> MKKEK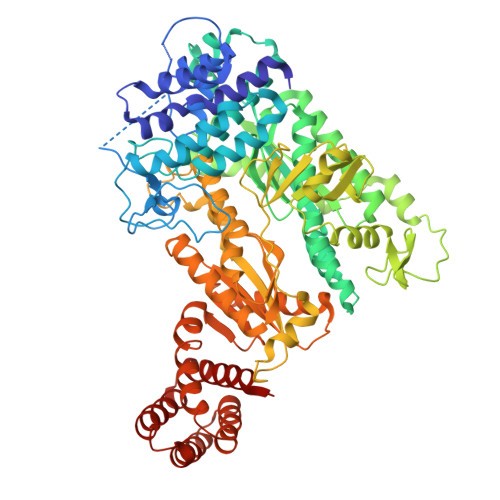IDLFYGALLHDIGKVIQRATGERKKHALVGADWFDEIADNQVISDQIRYHMANYQSDKLGNDHLAYITYIADNIASGVDRRQSNEESDEDTSAKIWDTYTNQADIFNVFGAQTDKRYFKPTVLNLKSKPNFASATYEPFSKGDYAAIATRIKNELAEFEFNQVQIDSLLNLFEATLSFVPSSTNTKEIADISLADHSRLTAAFALAIYDYLEDKGRHNYKEDLFTKVSAFYEEEAFLLASFDLSGIQDFIYNINIATNGAAKQLKARSLYLDFMSEYIADSLLDKLGLNRANMLYVGGGHAYFVLANTEKTVETLVQFEKDFNQFLLANFQTRLYVAFGWGSFAAKDIMSELNSPESYRQVYQKASRMISKKKISRYDYQTLMLLNRGGKSSERECEICHSVENLVSYHDQKVCDICRGLYQFSKEIAHDHFIITENEGLPIGPNACLKGVAFEKLSQEAFSRVYVKNDYKAGTVKATHVFVGDYQCDEIYNYAALSKNENGLGIKRLAVVRLDVDDLGAAFMAGFSQQGNGQYSTLSRSATFSRSMSLFFKVYINQFASDKKLSIIYAGGDDVFAIGSWQDIIAFTVELRENFIKWTNGKLTLSAGIGLFADKTPISLMAHQTGELEEAAKGNEKDSISLFSSDYTFKFDRFITNVYDDKLEQIRYFFNHQDERGKNFIYKLIELLRNHDRMNMARLAYYLTRLEELTRETDRDKFKTFKNLFYSWYTNKNDKDRKEAELALLLYIYEIRKD>MNQQLIETLKSKEGKMIEIRRYLHQHPELSFHEDETAKYIAEFYKGKDVEVETNVGPRGIKVTIDSGKPGKTLAIRADFDALPITEDTGLSFASQNKGVMHACGHDAHTAYMLVLAETLAEMKDSFTGKVVVIHQPAEEVPPGGAKTMIENGVLDGVDHVLGVHVMSTMKTGKVYYRPGYVQTGRAFFKLKVQGKGGHGSSPHMANDAIVAGSYFVTALQTVVSRRLSPFETGVVTIGSFDGKGQFNVIKDVVEIEGDVRGLTDATKATIEKEIKRLSKGLEDMYGVTCTLEYNDDYPALYNDPEFTEYVAKTLKEANLDFGVEMCEP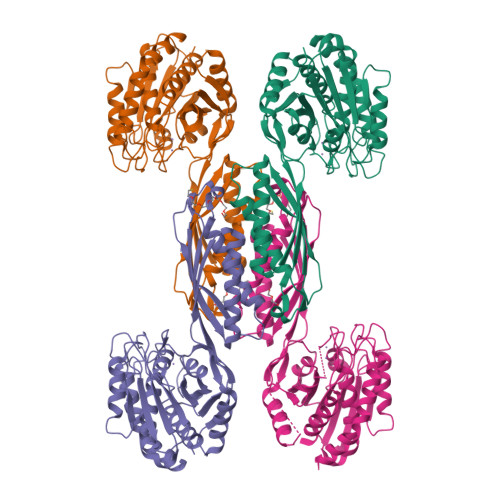QPPSEDFAYYAKERPSAFIYTGAAVENGEIYPHHHPKFNISEKSLLISAEAVGTVVLDYLKGDN[4x]>EAVVISGRKLAQQIKQEVRQEVEEWVASGNKRPHLSVILVGENPASHSYVLNKTRAAAVVGINSETIMKPASISEEELLNLINKLNNDDNVDGLLVQLPLPEHIDERRICNAVSPDKDVDGFHVINVGRMCLDQYSMLPATPWGVWEIIKRTGIPTLGKNVVVAGRSKNVGMPIAMLLHTDGAHERPGGDATVTISHRYTPKEQLKKHTILADIVISAAGIPNLITADMIKEGAAVIDVGINRVHDPVTAKPKLVGDVDFEGVRQKAGYITPVPGGVGPMTVAMLMKNTIIAAKKVLRLEEREVLKSKELGVATN[2x]

MTHFD2, a one-carbon metabolism enzyme, is localized in the mitochondria and plays an important role in nucleic acid biosynthesis, amino acid metabolism, and protein synthesis. It is a NAD-dependent enzyme and functions as both 5,10-methylenetetrahydrofolate (CH2-THF) dehydrogenase and 5,10-methenyltetrahydrofolate (CH+-THF) cyclohydrolase, converting CH2-THF to 10-formyl-THF (CHO-THF). MTHFD2 forms a homodimer and each monomer consists of the N-lobe and C-lobe connected by two long α helices. The MTHFD2 gene is upregulated in various cancers but very low or undetectable in normal proliferating cells, and therefore a potential target for cancer treatment.

Compound 9 and 15 show similar activities, despite having different chemical structures and, in particular, different tail moieties: whereas 15 bears a bulky glutamic moiety, 9 carries a relatively small propanoic moiety. To compare the interactions of these two compounds with MTHFD2, the structure of MTHFD2 in complex with 9 was solved to 2.25 Å (the ternary structure is hereafter referred to as MTHFD2/9/21) and compared with the MTHFD2/15/21 structure previously obtained. The propanoic acid group of 9 occupied a similar position to the γ-carboxyl group of glutamic acid in 15. However, the α-carboxyl group of 15 is absent in 9 and thus loses the hydrogen interaction network with Ser81, Gln132, and Leu133. Also, the core of 9 was observed to be shifted away from helix D, resulting in the loss of a hydrogen bond with Arg142. In addition, instead of direct interactions with Glu141 of MTHFD2 as observed with 15, 9 was found to interact with Glu141 through a water molecule. 9 and 15 also have different head moieties: whereas, 15 bears a phenyl-based head, 9 has an indole moiety consisting of two fused rings. The indole moiety was found to extend further into the dimer interface compared to the phenyl-based head, leading to the formation of stronger shape complementarity interactions with MTHFD2 and the additional hydrophobic interactions with Lys203 and Met207. Most importantly, the nitrogen atom on the indole moiety of 9 was hydrogen bonded with the side chain of Asn204, which is absent in the structure of 15 bound to MTHFD2. The more extensive shape complementarity interactions and the additional hydrogen-bond interaction around the head group of 9 compensate for the losses of hydrogen-bond networks observed in the tail group of 15, resulting in the comparable activity of these two inhibitors.>[2x]GSPEKILAQIIQEHREGLDWQEAATRASLSLEETRKLLQSMAAAGQVTLLRVENDLYAISTERYQAWWQAVTRALEEFHSRYPLRPGLAREELRSRYFSRLPARVYQALLEEWSREGRLQLAANTVALAGFTPS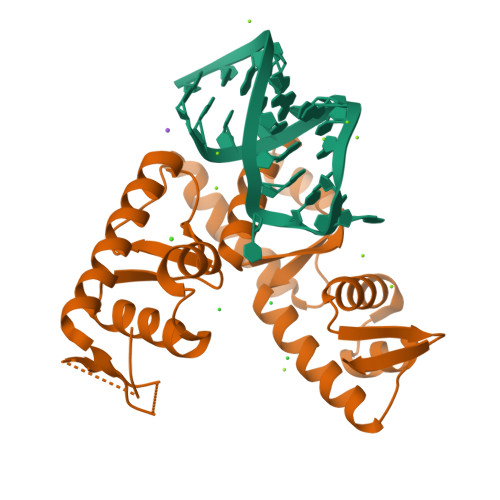FSETQKKLLKDLEDKYRVSRWQPPWVKEVAGSFNLDPSELEELLHYLVREGVLVKINDEFYWHRQALGEAREVIKNLASTGPFGLAEARDALGSSRKYVLPLLEYLDQVKFTRRVGDKRVVVGN> MGHPEIVAAAVAFVRQIW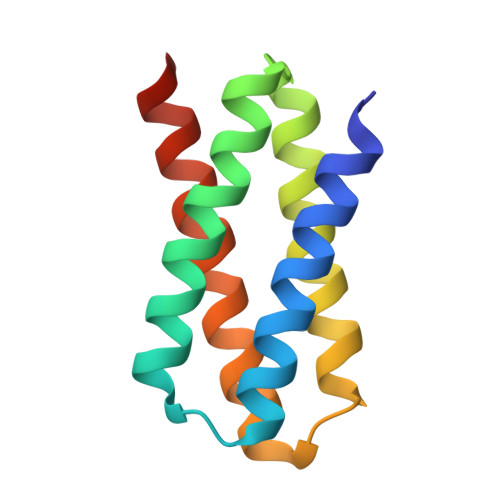EYARQGMSLDEMIAWAVKYAKKIFDLVKKMGASDEVLKKVMDAVLAAAQAYAQQLNDEAAQRLLVAAQVIVQVLQQLGLEHHHHHH> LNNLQNIIYNPVIPFVGTIPDQLDPGTLIVIRGHVPSDADRFQVDLQNGSSM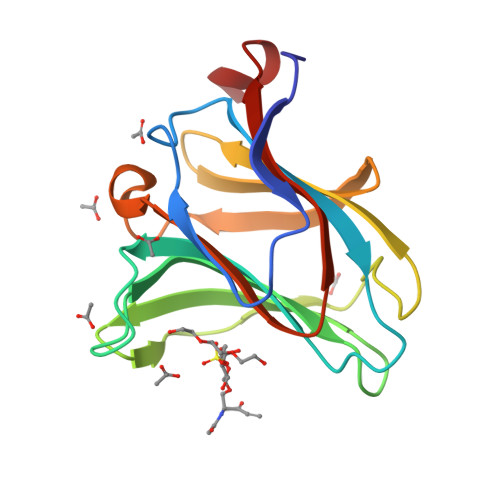KPRADVAFHFNPRFKRAGCIVCNTLINEKWGREEITYDTPFKREKSFEIVIMVLKDKFQVAVNGKHTLLYGHRIGPEKIDTLGIYGKVNIHSIGFSFSSDLQST> MGSSHHHHHHSSGLVPRGSMTLPAFKAYDIRGRVPDELNEDLARRIGVALAAQLDQGPVVLGHDVRLASPALQEALSAGLRASGRDVIDIGLCGTEEVYFQTDYLKAAGGVMVTASHNPMDYNGMKLVREQARPISSDTGLFAIRDTVAADTAAPGEPTASEQSRTDKTAYLEHLLSYVDRSTLKPLKLVVNAGNGGAGLIVDLLAPHLPFEFVRVFHE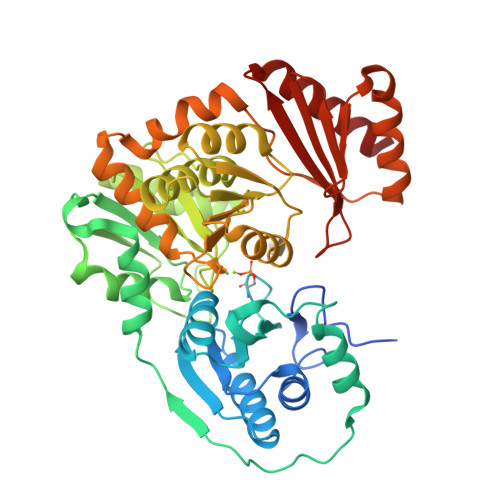PDGNFPNGIPNPLLPENRDATAKAVKDNGADFGIAWDGDFDRCFFFDHTGRFIEGYYLVGLLAQAILAKQPGGKVVHDPRLTWNTVEQVEEAGGIPVLCKSGHAFIKEKMRSENAVYGGEMSAHHYFREFAYADSGMIPWLLIAELVSQSGRSLADLVEARMQKFPCSGEINFKVADAKASVARVMEHYASLSPELDYTDGISADFGQWRFNLRSSNTEPLLRLNVETRGDAALLETRTQEISNLLRG>[2x]MISLADLQRRIETGELSPNAAIAQSHAAIEAREKEVHAFVRHDK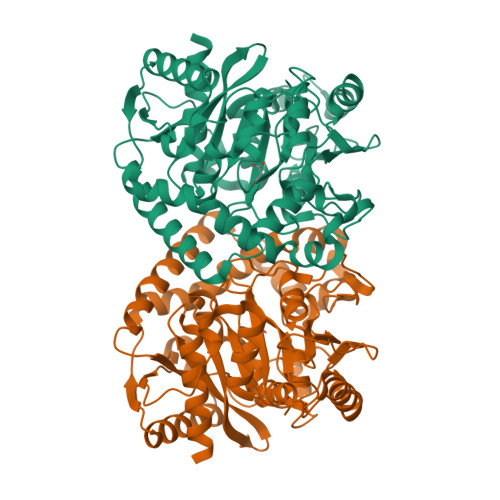SARAQASGPLRGIAVGIKDIIDTANMPTEMGSEIYRGWQPRSDAPVVMMLKRAGATIIGKTTTTAFASRDPTATLNPHNTGHSPGGASSGSAAAVGAGMIPLALGTQTGGSVIRPAAYCGTAAIKPSFRMLPTVGVKCYSWALDTVGLFGARAEDLARGLLAMTGRSEFSGIVPAKAPRIGVVRQEFAGAVEPAAEQGLQAAIKAAERAGASVQAIDLPEAVHEAWRIHPIIQDFEAHRALAWEFSEHHDEIAPMLRASLDATVGLTPKEYDEARRIGRRGRRELGEVFEGVDVLLTYSAPGTAPAKALASTGDPRYNRLWTLMGNPCVNVPVLKVGGLPIGVQVIARFGNDAHALATAWFLEDALAKSG> KILHR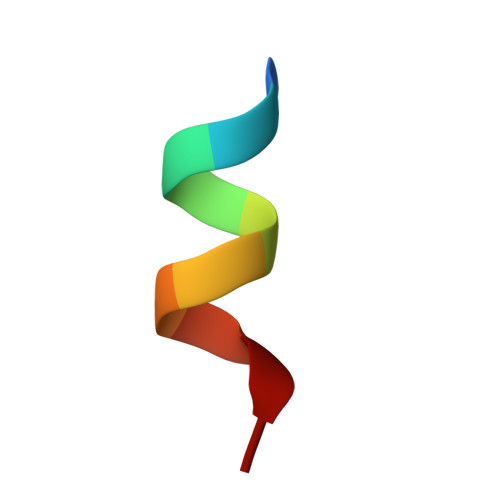LLQDS>[3x]GSTDPNI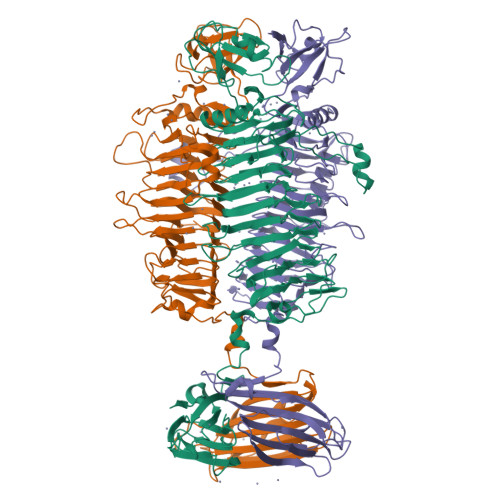DMTKWVKSTDSVQVDSVNALRKVKGLFHNQKATTTSYVAGTGFGGATYLWDANNTATDDGLSVIRVTGAATGAWLLQVHNKVLHATQAGLRAELLESDLIDQTTILQKCVDYMALIGGGVVQLPKGHIYAKAMAKSNVEVRGTFDSFVSVGSEADINNLRTVVQTATYKHGTFWHSSDGSQVYLVPENVTGAGVSNLKMLGSRLGSTSSNCGFGIKIIGDSFTAKWVDTSGFRLEGLYIRGKDGVSCSNHYFENCNFLDARRNTAALVYCHDVTFKNCTFQQLKPELTWVYLFDIEPNPATTDTVYNVTLINCVFNALASAGAEPTVLVKEQNTPTGSPNVKFLNCRFKGKATIRNNCANGWKDCIVDNCEFDTLAFSTTTTGYVITSGRFTNNTLWGKDLKGFSYNTLVTGDFLIEGNRFQDTTFENNIVATQASFGVNTFLGTATVIQPVDRRTITQQYRNLPDISGVKSPINDAYFNTEIRNFNLDLNFKEVLTVPLRSGCKITITGADATTNAGSKAYVELFVNSDNSTTITAHNEVINDPLYGVKYSWSGRTLSLAGITLSANTFIVKVDVFSALPQYSKVTWLI>MANVIKTVLTYQLDGSNRDFNIPFEYLARKFVVVTLIGVDRKVLTINTDYRFATRTTISLTKAWGPADGYTTIELRRVTSTTDRLVDFTDGSI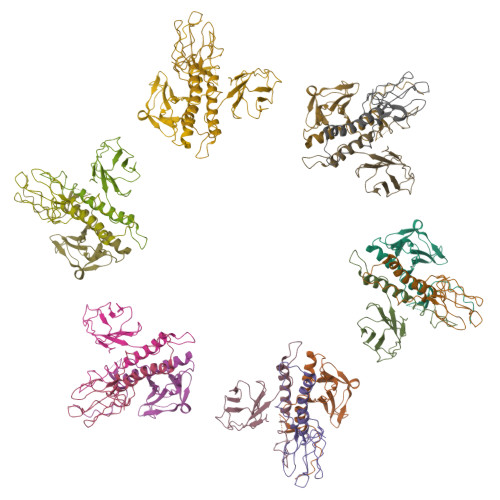LRAYDLNVAQIQTMHVAEEARDLTTDTIGVNNDGHLDARGRRIVNLANAVDDRDAVPFGQLKTMNQNSWQARNEALQFRNEAETFRNQAEGFKNESSTNATNTKQWRDETKGFRDEAKRFKNTAGQYATSAGNSASAAHQSEVNAENSATASANSAHLAEQQADRAEREADKLENYNGLAGAIDKVDGTNVYWKGNIHANGRLYMTTNGFDCGQYQQFFGGVTNRYSVMEWGDENGWLMYVQRREWTTAIGGNIQLVVNGQIITQGGAMTGQLKLQNGHVLQLESASDKAHYILSKDGNRNNWYIGRGSDNNNDCTFHSYVHGTTLTLKQDYAVVNKHFHVGQAVVATDGNIQGTKWGGKWLDAYLRDSFVAKSKAWTQVWSGSAGGGVSVTVSQDLRFRNIWIKCANNSWNFFRTGPDGIYFIASDGGWLRFQIHSNGLGFKNIADSRSVPNAIMVENE[18x]The highly up-regulated CJA_3010 encodes a signal peptidase II lipoprotein signal peptide (predicted by LipoP 1.0), followed by a serine-rich linker and a GH5_4 catalytic module, and was thus predicted to be anchored extracellularly in the outer membrane by N-terminal cysteine lipidation. Indeed CjGH5D, CjGH5E, and CjGH5F all displayed high specific activity toward XyG. The limit-digest products further revealed that all C. japonicus GH5_4 enzymes specifically catalyze hydrolysis at the anomeric position of the unbranched glucose residues of the (galacto)XyG polysaccharide chain. The overall structure of CjGH5D (residues Gly96 to Gln468) is an (β/α)8 barrel as is typical for GH5 family members.

A time- and concentration-dependent inactivation of the enzyme CjGH5D was observed upon incubation with XXXG-NHCOCH2Br, which followed pseudo-first-order kinetics. The dissociation constant Ki and the irreversible inactivation constant ki for XXXG-NHCOCH2Br towards CjGH5D were 1.78 ± 0.17 mM and 0.17 ± 0.01 min−1, respectively, resulting in a ki/Ki value (9.3 × 10−2 mM−1 min−1) that was comparable to that previously observed for a Prevotella bryantii GH5_4 member (PbGH5A). Notably, intact protein mass spectrometry of CjGH5D following incubation with the inhibitor indicated covalent labelling with 1:1 stoichiometry and no over-labelling of the enzyme. A second oligosaccharide complex was obtained at 2.1 Å resolution by soaking CjGH5D crystals with the N-bromoacetyl affinity label XXXG-NHCOCH2Br, in which the reagent had indeed reacted through attack of the catalytic general acid/base sidechain to displace the bromide nucleofuge. In molecule A of the asymmetric unit, there is electron density for GXXG-NHCOCH2-CjGH5D, whilst in molecule B, XXXG-NHCOCH2-CjGH5D is modeled, but with the − 3′- and − 4′-xylosyl sugars modelled at half occupancy. The carboxyl oxygen of the N-acetyl moiety forms a hydrogen bond with His323. There are hydrogen bonds between this subsite − 1 sugar and the catalytic nucleophile Glu390, and also to His208 and Asn254. The covalent adduct formation through the reactivity of the N-bromoacetyl reagent is fascinating given that in the structures observed here, the attack is made by the acid–base Glu255, as opposed to the enzymatic nucleophile of the enzymatic reaction, Glu390. However, Glu390 is too distant (6–7 Å) from the reactive carbon of the N-bromoacetyl moiety, and has impossible geometry and steric hindrance, to permit nucleophilic interception. The reactive group, however, is located in the + 1 subsite—some 3.8 Å from C1—thus can be fortuitously attacked by the acid/base which is in almost ideal position for SN2 attack on the reactive carbon to displace the bromide.

>MGSSHHHHHHSSGLVPRGSHMASGLYPSYNTSPAAPDSTGMQSTAVQLAGKIRLGWNIGNTMEAIGGETAWGNPMVSNELLKLVKDSGFDAVRIPVAWDQYANQESAEISAAWLNRVKQVVQMAIDNELYVLINIHWDGGWLENNITPAKKDENNAKQKAFWEQIATHLRDFDEHLLFAGTNEPNAENAEQMDVLNSYLQTFVDAVRSTGGKNAYRVLVLQGPVTDIEKTNELWTHMPADTATDRLMAEVHFYTPYNFALMRQDESWGKQFYYWGEGFLSTTDTERNPTWGEEATIDQLFDLMKTKFVDQGIPVVLGEFSAMRRTNLTGDALTLHLAGRAYYHKYVTQQALARGLLPFYWDNGGNDNFSSGIFNRQQNTVFDQQVLDALLEGAGAQ[2x]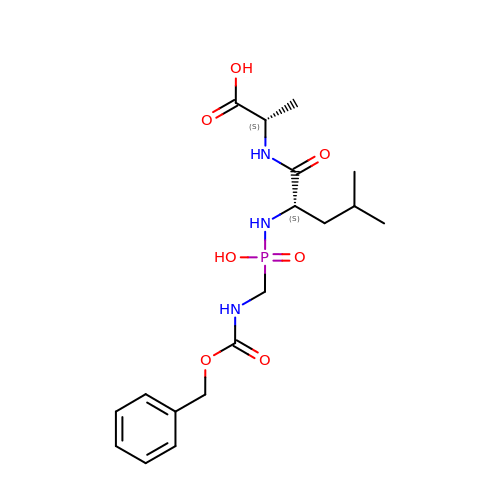N-[(S)-({[(benzyloxy)carbonyl]amino}methyl)(hydroxy)phosphoryl]-L-leucyl-L-alanine | C18 H28 N3 O7 P | DVNAMUNBHDIPLR-ZFWWWQNUSA-N>[2x]GHHHHHHEFMHVFDNNGIELKAECSIGEEDGVYGLILESWGPGDRNKDYNIALDYIIERLVDSGVSQVVVYLASSSVRKHMHSLDERKIHPGEYFTLIGNSPRDIRLKMCGYQAYFSRTGRKEIPSGNRTKRILINVPGIYSDSFWASIIRG

EcoKMcrA from Escherichia coli restricts CpG methylated or hydroxymethylated DNA, and may act as a barrier against host DNA. The enzyme consists of a novel N-terminal specificity domain that we term NEco, and a C-terminal catalytic HNH domain. We determined the crystal structures of NEco in complex with fully modified DNA containing three variants of the Y5mCGR EcoKMcrA target sequence: C5mCGG, T5mCGA and T5hmCGA. The structures show that monomeric NEco has two separate pockets for (hydroxy)methyl groups on cytosines, reachable without nucleotide flipping, and reveal the mechanistic basis for the Y5(h)mCGR sequence specificity of EcoKMcrA.

The purified NEco was co-crystallized with 10mer dsDNA with the central C5mCGG, T5mCGA and T5hmCGA sequences. The protein potently restricts methylated and hydroxymethylated DNA (from the glucosyltransferase deficient T4gt or T6gt phage), but not glucosyl-hydroxymethylated DNA (from wild-type T4 phage). However, the enzyme is also effective against hydroxymethylated DNA (unless it is further glucosylated). The structure with T5hmCGA DNA readily explains this observation. In both proximal and distal strands, the hydroxymethyl groups are accommodated in the respective pockets and form direct hydrogen bonds with the protein backbone. A hydroxymethyl group is also tolerated in this position, and donates a hydrogen bond to the main chain carbonyl of G34. We also find that NEco has a significant (∼40-fold) preference for fully methylated over fully hydroxymethylated DNA, and intermediate affinity to hybrid methylated/hydroxymethylated DNA. Nevertheless, the remaining affinity to fully hydroxymethylated DNA must be sufficient for restriction. The protein-DNA complexes in the three NEco structures are highly similar (all atom rmsd between 0.3 and 0.9 Å).{1-(ethylsulfonyl)-3-[4-(2-{[4-(1-methylpiperidin-4-yl)phenyl]amino}-7H-pyrrolo[2,3-d]pyrimidin-4-yl)-1H-pyrazol-1-yl]azetidin-3-yl}acetonitrile | C28 H33 N9 O2 S 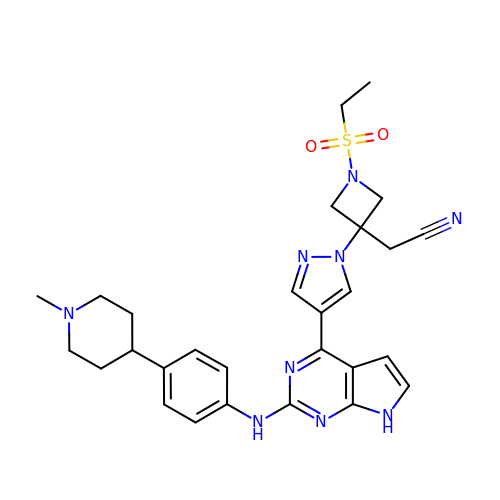| VEXRNZJDEGTDGD-UHFFFAOYSA-N>[2x]GSHMSDLPLRFPYGRPEFLGLSQDEVECSADHIARPILILKETRRLPWATGYAEVINAGKSTHNEDQASCEVLTVKKKAGAVTST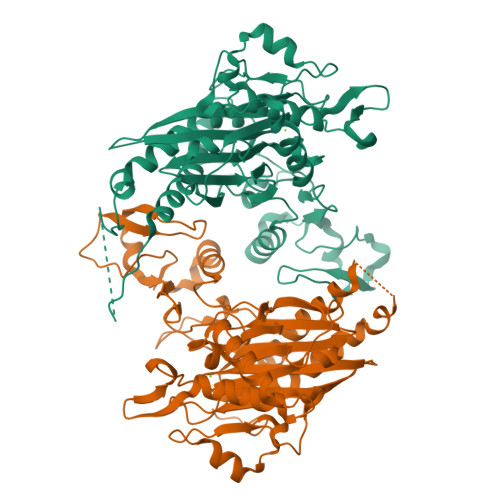PNRNSSKRRSSLPNGEGLQLKENSESEGVSCHYWSLFDGHAGSGAAVVASRLLQHHITEQLQDIVDILKNSAVLPPTCLGEEPENTPANSRTLTRAASLRGGVGAPGSPSTPPTRFFTEKKIPHECLVIGALESAFKEMDLQIERERSSYNISGGCTALIVICLLGKLYVANAGASRAIIIRNGEIIPMSSEFTPETERQRLQYLAFMQPHLLGNEFTHLEFPRRVQRKELGKKMLYRDFNMTGWAYKTIEDEDLKFPLIYGEGKKARVMATIGVTRGLGDHDLKVHDSNIYIKPFLSSAPEVRIYDLSKYDHGSDDVLILATDGLWDVLSNEEVAEAITQFLPNCDPDDPHRYTLAAQDLVMRARGVLKDRGWRISNDRLGSGDDISVYVIPLIHGNKLS> MFSAGHKIKGTVVLMPKNELEVNPDGSAVDNLNAFLGRSVSLQLISATKADAHGKGKVGKDTFLEGINTSLPTLGAGESAFNIHFEWDGSMGIPGAFYIKNYMQVEFFLKSLTLEAISNQGTIRFVCNSWVYNTKLYKSVRIFFANHTYVPSETPAPLVEYREEELKSLRGNGTG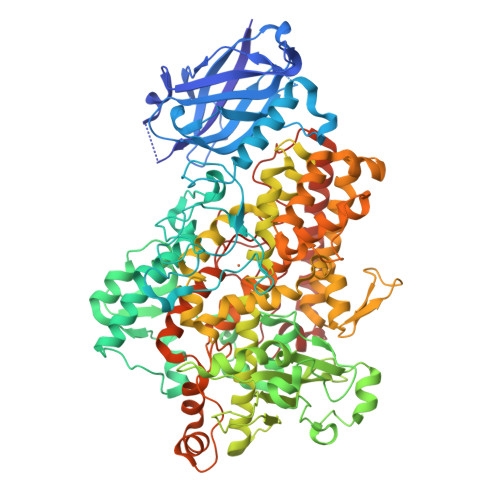ERKEYDRIYDYDVYNDLGNPDKSEKLARPVLGGSSTFPYPRRGRTGRGPTVTDPNTEKQGEVFYVPRDENLGHLKSKDALEIGTKSLSQIVQPAFESAFDLKSTPIEFHSFQDVHDLYEGGIKLPRDVISTIIPLPVIKELYRTDGQHILKFPQPHVVQVSQSAWMTDEEFAREMIAGVNPCVIRGLEEFPPKSNLDPAIYGDQSSKITADSLDLDGYTMDEALGSRRLFMLDYHDIFMPYVRQINQLNSAKTYATRTILFLREDGTLKPVAIELSLPHSAGDLSAAVSQVVLPAKEGVESTIWLLAKAYVIVNDSCYHQLMSHWLNTHAAMEPFVIATHRHLSVLHPIYKLLTPHYRNNMNINALARQSLINANGILETTFLPSKYSVEMSSAVYKNWVFTDQALPADLIKRGVAIKDPSTPHGVRLLIEDYPYAADGLEIWAAIKTWVQEYVPLYYARDDDVKNDSELQHWWKEAVEKGHGDLKDKPWWPKLQTLEDLVEVCLIIIWIASALHAAVNFGQYPYGGLIMNRPTASRRLLPEKGTPEYEEMINNHEKAYLRTITSKLPTLISLSVIEILSTHASDEVYLGQRDNPHWTSDSKALQAFQKFGNKLKEIEEKLVRRNNDPSLQGNRLGPVQLPYTLLYPSSEEGLTFRGIPNSISI> MAHHHHHHSAALEVLFQGPGMASGSNVEEYELDVEALVVILRDRNIPRNPLHGEVIGLRLTEGWWGQIERFQMVRLILQNDDNEPLQRPRYEVIQRAVNPHTMFMISGPLAELQLAFQDLDLPEGPLRFGPLANGHYVQGDPYSSSYRPVTMAETAQMTRDELEDVLNTQSEIEIQMINLLELYEVETRALR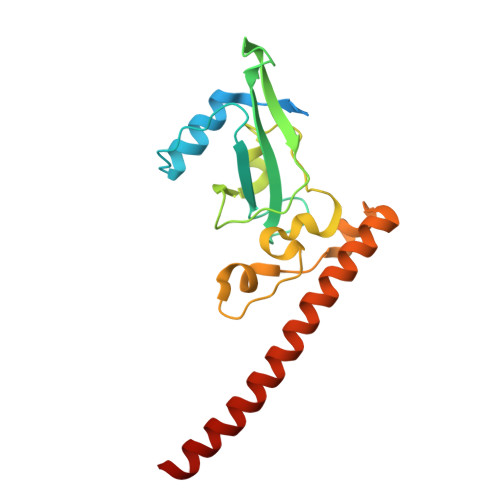RQLAERS> GARDVQEGVSSFEESGGAQLPPRVHALEVLEGAGPGRLHGRLGIKPDGQPGYTRAPSPPTDLSMPQALARGGGFNLYLSDHLELDRTAPDARHASCRQLHYDLSTLPKASVIIVFYNEPFSTLMRSVHSVLNGTPPQILEELILVDDGSTLPYIRE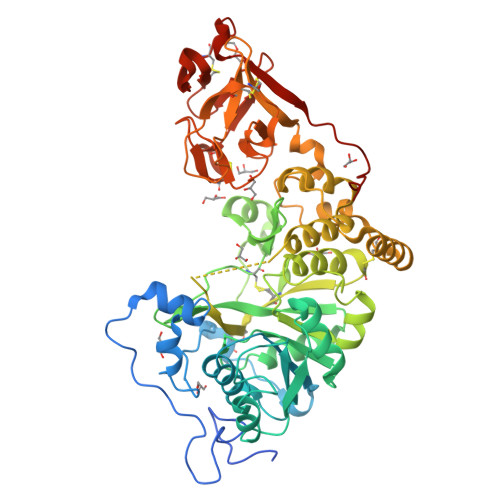DGNQQLVEYLKLLPAKVRLIRNEVRKGIVGARMKGIRASRAPIFAILDSHIEVSPQWLEPLLLRIKEDSRRVVMPQIDGIDAETFKHIAGGIGCKLGFLWKLMEHSYEGHQTARLPPEERQPSPTDFQTSPAMAGGLFAANKAFFFDVGAYDEDFQFWGTENLELSFRLWQCGGVLECAPCSRVYHIFRKGGSGYSSPGDSITINKMRTMLWMDEYADLAWRVIGKPRVNYRPESLEKRREWRKRKGCKSFRWFMENVFPEGDVVTLDDVPYLGPLRNDKIGMCLDNMGWASPGHAVGLEYCHGGDTQTFMFFRKVGHVMPVNDDEACLQPSGRLDWCRGTAQFWWDFTSSGQLMFRETKQCLSAFGRKLRMVECDDTDPYQIWSWTAYNPPDTFTFPSVSRSIRSG propane-1-thiol 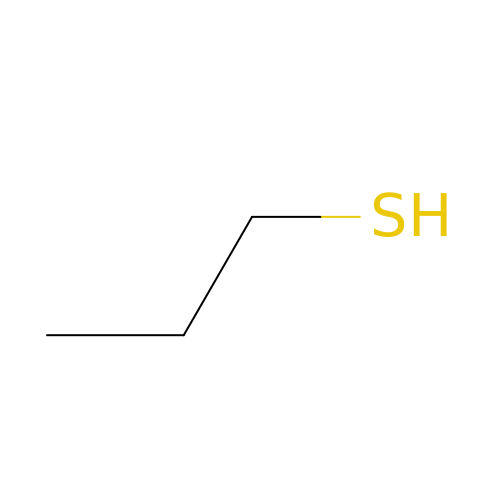| C3 H8 S | SUVIGLJNEAMWEG-UHFFFAOYSA-N ethyl (2R,3S)-3-(5-bromopyridin-2-yl)-2-fluoro-3-hydroxypropanoate 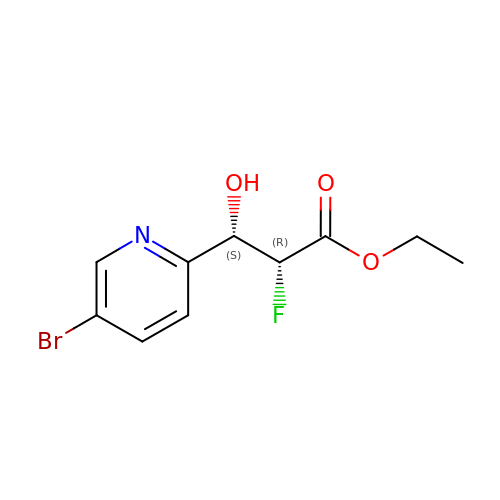| C10 H11 Br F N O3 | JAJULJUIZXJSOC-BDAKNGLRSA-N> MKHHHHHHPMAPAPVAQVKVIFTTTEPDLELPESKRQLLVPADIR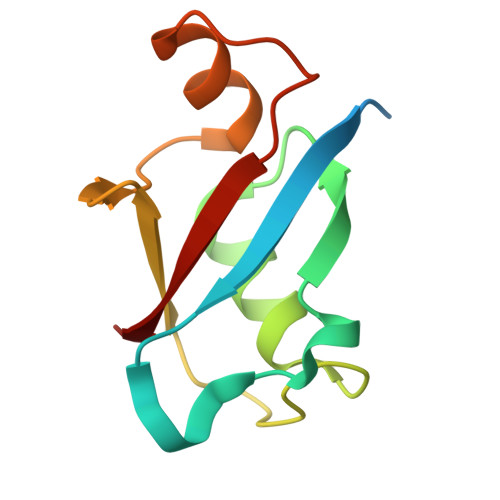RYGLSRILNSESMLDTGSIPFDFLINGSFLRSSLEDYLTSNGLSLETTLTLQYVRS Rhino- and enteroviruses (family Picornaviridae) are important human pathogens. The best studied inhibitors are the so-called “capsid binders” (such as pleconaril, pirodavir, vapendavir, and pocapavir). These compounds fit in a hydrophobic pocket in the viral particle, thereby preventing binding of the virus to the receptor and/or uncoating. Now 32 years after its discovery, we report on a novel druggable pocket within a conserved VP1-VP3 interprotomer interface of the viral capsid.

To gain insights into the interaction of the drug with the viral capsid, a 4.0-Å structure of the CVB3–compound 17 complex was determined by cryo–electron microscopy (EM) and image reconstruction. However, difference map analysis revealed additional density that could easily be fitted with an atomic model of compound 17. The compound has an L-shaped structure with a longer and a shorter arm, allowing unambiguous docking. Modelling revealed that compound 17 binds into a pocket formed by two VP1 units and one VP3 unit at an interprotomer interface. Because of the icosahedrally symmetric nature of the virus, there are 60 such sites in one capsid, with 5 around each 5-fold vertex. This interprotomer site is 16 Å away from the hydrophobic pocket targeted by pleconaril and other capsid inhibitors, raising the possibility of complementary antiviral effects (for those strains susceptible to both classes of compounds). The cryo-EM structure indicates that there is charge complementarity between R3 and the conserved residue VP1_R234. Hence, we propose that binding of compounds in this pocket stabilizes the conformation of a key region of the virion, preventing rearrangements that allow transition to the A-particle.

> GPVEDAITAAIGRVADTVGTGPTNSEAIPALTAAETGHTSQVVPGDTMQTRHVKNYHSRSESTIENFLCRSACVYFTEYKNSGAKRYAEWVLTPRQAAQLRRKLEFFTYVRFDLELTFVITSTQQPSTTQNQDAQILTHQIMYVPPGGPVPDKVDSYVWQTSTNPSVFWTEGNAPPRMSIPFLSIGNAYSNFYDGWSEFSRNGVYGINTLNNMGTLYARHVNAGSTGPIKSTIRIYFKPKHVKAWIPRPPRLCQYEKAKNVNFQPSGVTTTRQSITTMTNTGAF;> SPTVEECGYSDRARSITLGNSTITTQECANVVVGYGVWPDYLKDSEATAEDQPTQPDVATCRFYTLDSVQWQKTSPGWWWKLPDALSNLGLFGQNMQYHYLGRTGYTVHVQCNASKFHQGCLLVVCVPEAEMGCATLDNTPSSAELLGGDTAKEFADKPVASGSNKLVQRVVYNAGMGVGVGNLTIFPHQWINLRTNNSATIVMPYTNSVPMDNMFRHNNVTLMVIPFVPLDYCPGSTTYVPITVTIAPMCAEYNGLRLAGHQ;> GLPTMNTPGSCQFLTSDDFQSPSAMPQYDVTPEMRIPGEVKNLMEIAEVDSVVPVQNVGEKVNSMEAYQIPVRSNEGSGTQVFGFPLQPGYSSVFSRTLLGEILNYYTHWSGSIKLTFMFCGSAMATGKFLLAYSPPGAGAPTKRVDAMLGTHVIWDVGLQSSCVLCIPWISQTHYRFVASDEYTAGGFITCWYQTNIVVPADAQSSCYIMCFVSACNDFSVRLLKDTPFISQQNFFQ;> MGAQVSTQKTGAHETRLNASGNSIIHYTNINYYKDAASNSANRQDFTQDPGKFTEPVKDIMIKSLPALN> HKKLLQLL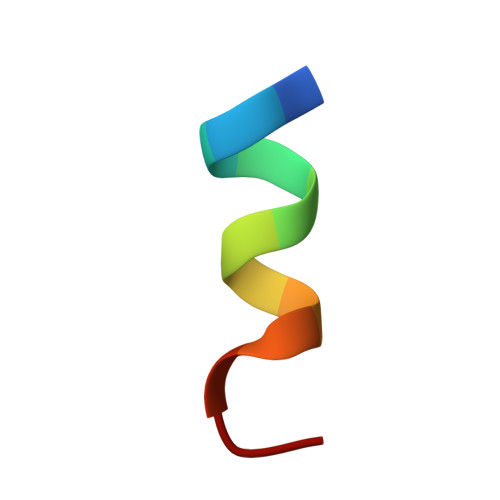TCSS> MSGVRAVRISIESACEKQVHEVGLDGTETYLPPLSMSQNLARLAQRIDFSQGSGSEEEEAAGTEGDAQEWPGAGSSADQDDEEGVVKFQPSLWPWDSVRNNLRSALTEMCVLYDVLSIVRDKKFMTLDPVSQDALPPKQNPQTLQLISKKKSLAGAAQILLKGAERLTKSVTENQENKLQRDFNSELLRLRQHWKLRKVGDKILGDLSYRSAGSLFPHHGTFEVIKNTDLDLDKKIPEDYCPLDVQIPSDLEGSAYIKVSIQKQAPDIGDLGTVNLFKRPLPKSKPGSPHWQTKLEAAQNVLLCKEIFAQLSREAVQIKSQVPHIVVKNQIISQPFPSLQLSISLCHSSNDKKSQKFATEKQCPEDHLYVLEHNLHLLIREFHKQTLSSIMMPHPASAPFGHKRMRLSGPQAFDKNEINSLQSSEGLLEKIIKQAKHIFLRSRAAATIDSLASRIEDPQIQAHWSNINDVYESSVKVLITSQGYEQICKSIQLQLNIGVEQIRVVHRDGRVITLSYQEQELQDFLLSQMSQHQVHAVQQLAKVMGWQVLSFSNHVGLGPIE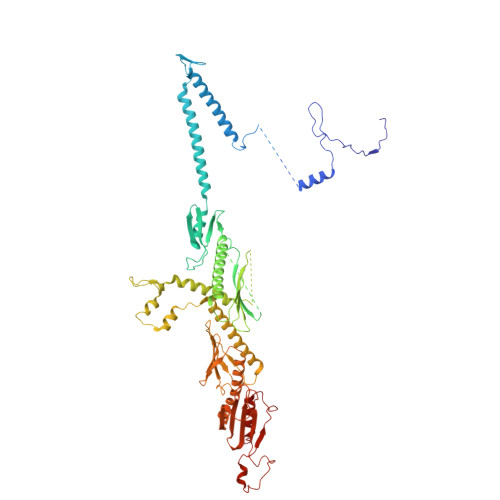SIGNASAITVASPSGDYAISVRNGPESGSKIMVQFPRNQCKDLPKSDVLQDNKWSHLRGPFKEVQWNKMEGRNFVYKMELLMSALSPCLL(3~{R})-3-methyl-2-oxidanylidene-pentanedioic acid | C6 H8 O5 | 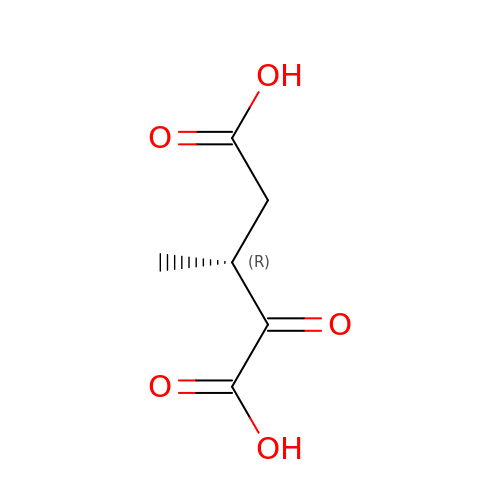BJQIUPTURRAODO-GSVOUGTGSA-N> ARKL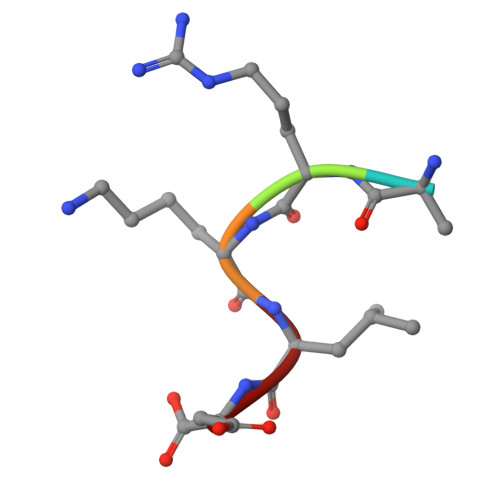D>[4x]MGSDKIHHHHHHENLYFQGMKITTKGRYGLTITLELAKRIGDGPISLRSIAQD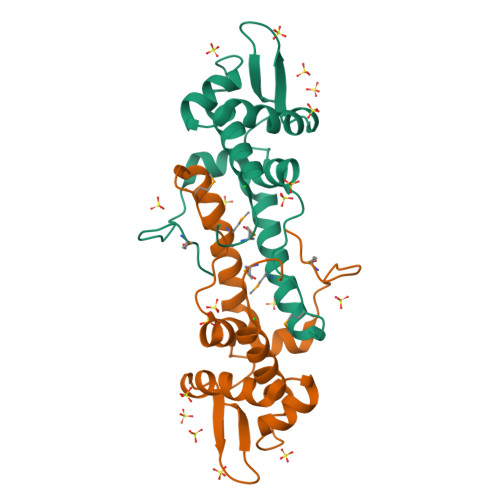KNLSEHYLEQLIGPLRNAGIVKSIRGAHGGYVLNGDPEKITAGDIIRTLEGPIVLVESMEDEEAAQRELWTRMRNAVRDVLDQTTLSDLLKHSTDSELTDGYMFYI> ENKCIAVNENKVIENQKVIQSLCKNSHLDLIEQSYFGECDFIINHSTCVYKIQASRFMQLRNNGSLHYDKAVNDLLTEFQRVIIIVEFSEIIQDVD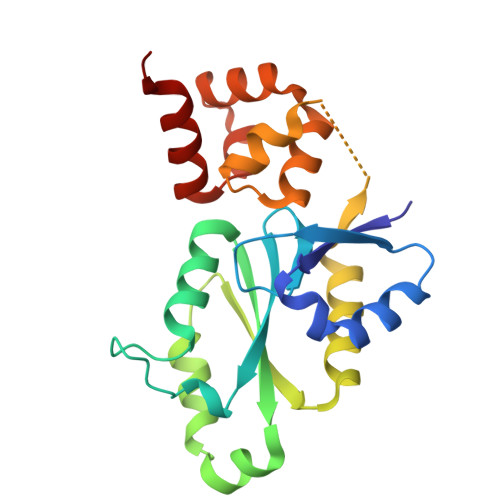PDLFWKIKLYLLNSRVDVFFIHETTDFFIDWMKYFIARWAFSYNDEAAANIANADILLDLGFNILLVRKIFQTYSLEEFFMAIIKEESKAVKMLTVSQMTRLKKLLTLEW>[8x]SNAVAVSSKIDTEGGVLGNIILTVLNANGIKTTDRIQLGATPVVR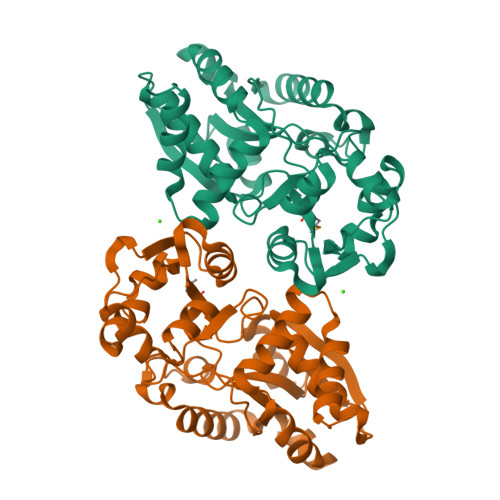KAITAGEIDIYPEYTGNAAFFFNKADDPLWKDPAKAYETAKKLDYDANKIVWLTPSPANNTWGIAVRKDVANENKLASLSDFGKYIAGGGKVVLAASSEFVNSAAALPAFQTAYGFTLKPDQLITLSGGDTAATIAAAANQTNGANAAMVYGTDGGIAPSGLVVLEDDKHVQPVYQPAPIIREEVLKKDPKIEELLKPVFEKLDLTTLQDLNGRVQLGGEPAKAVAEDFLKKNGFLK>ARVAVLISGTGSNLQALIDSTREPNSSAQIDIVISNKAAVAGLDKAERAGIPTRVINHKLYKNRVEFDSAIDLVLEEFSIDIVCLAGFMRILSGPFVQKWNGKMLNIHPSLLPSFKGSNAHEQALETGVTVTGCTVHFVAEDVDA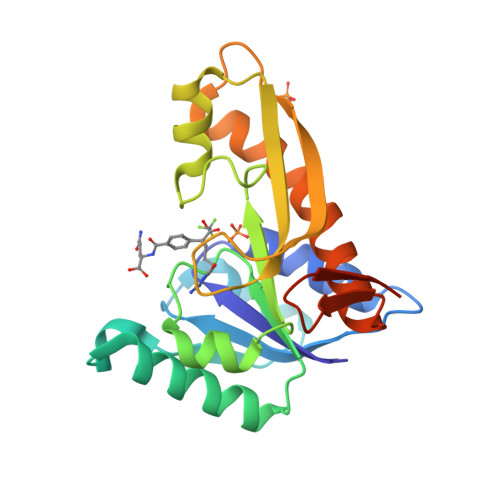GQIILQEAVPVKRGDTVATLSERVKLAEHKIFPAALQLVASGTVQLGENGKICWVKEEHHHHHH[2x]> MLKRKQSSRVEAQPVTDFGPDESLSDNADILWINKPWVHSLLRICAIISVISVCMNTPMTFEHYPPLQYVTFTLDTLLMFLYTAEMIAKMHIRGIVKGDSSYVKDRWCVFDGFMVFCLWVSLVLQVFEIADIVDQMSPWGMLRIPRPLIMIRAFRIYFRFELPRTRITNILKRSGEQIWSVSIFLLFFLLLYGILGVQMFGTFTYHCVVNDTKPGNVTWNSLAIPDTHCSPELEEGYQCPPGFKCMDLEDLGLSRQELGYSGFNEIGTSIFTVYEASSQEGWVFLMYRAIDSFPRWRSYFYFITLIFFLAWLVKNVFIAVIIETFAEIRVQFQQMWGTRSSTTSTATTQMFHEDAAGGWQLVAVDVNKPQGRAPACLQKMMRSSVFHMFILSMVTVDVIVAASNYYKGENFRRQYDEFYLAEVAFTVLFDLEALLKIWCLGFTGYISSSLHKFELLLVIGTTLHVYPDLYHSQFTYFQVLRVVRLIKISPALEDFVYKIFGPGKKLGSLVVFTASLLIVMSAISLQMFCFVEELDRFTTFPRAFMSMFQILTQEGWVDVMDQTLNAVGHMWAPLVAIYFILYHLFATLILLSLFVAVILDNLELDEDLKKLKQLKQSEANADTKEKLPLRLRIFEKFPNRPQMVKISKLPSDFTVPKIRESFMKQFIDRQQQDTCCLFRILPSTSSSSCDNPKRPTVEDNKYIDQKLRKSVFSIRARNLLEKETAVTKILRACTRQRMLSGSFEGQPAKERSILSVQHHIRQERRSLRHGSNSQRISRGKSLETLTQDHSNTVRYRNAQREDSEIKMIQEKKEQAEMKRKVQEEELRENHPYFDKPLFIVGREHRFRNFCRVVVRARFNASKTDPVTGAVKNTKYHQLYDLLGLVTYLDWVMITVTICSCISMMFESPFRRVMHAPTLQIAEYVFVIFMSIELNLKIMADGLFFTPTAVIRDFGGVMDIFIYLVSLIFLCWMPQNVPAESGAQLLMVLRCLRPLRIFKLVPQMRKVVRELFSGFKEIFLVSILLLTLMLVFASFGVQLFAGKLAKCNDPNIIRREDCNGIFRINVSVSKNLNLKLRPGEKKPGFWVPRVWANPRNFNFDNVGNAMLALFEVLSLKGWVEVRDVIIHRVGPIHGIYIHVFVFLGCMIGLTLFVGVVIANFNENKGTALLTVDQRRWEDLKSRLKIAQPLHLPPRPDNDGFRAKMYDITQHPFFKRTIALLVLAQSVLLSVKWDVEDPVTVPLATMSVVFTFIFVLEVTMKIIAMSPAGFWQSRRNRYDLLVTSLGVVWVVLHFALLNAYTYMMGACVIVFRFFSICGKHVTLKMLLLTVVVSMYKSFFIIVGMFLLLLCYAFAGVVLFGTVKYGENINRHANFSSAGKAITVLFRIVTGEDWNKIMHDCMVQPPFCTPDEFTYWATDCGNYAGALMYFCSFYVIIAYIMLNLLVAIIVENFSLFYSTEEDQLLSYNDLRHFQIIWNMVDDKREGVIPTFRVKFLLRLLRGRLEVDLDKDKLLFKHMCYEMERLHNGGDVTFHDVLSMLSYRSVDIRKSLQLEELLAREQLEYTIEEEVAKQTIRMWLKKCLKRIRAKQQQSCSIIHSLRESQQQELSRFLNPPSIETTQPSEDTNANSQDHNTQPESSSQQQLLSPTLSDRGGSRQDAADTGKPQRKIGQWRLPSAPKPISHSVSSVNLRFGGRTTMKSVVCKMNPMPDTASCGSEVKKWWTRQLTVESDESGDDLLDI;> MTRGAWMCRQYDDGLKIWLAAPRENEKPFIDSERAQKWRLSLASLLFFTVLLSDHLWFCAEAKLTRTRDKEHHQQQQQQQQQQQQQQQQQQQQQQRQQQRQRQQQRQRQQEPSWPALLASMGESSPAAQAHRLLSASSSPTLPPSPGGGGGSKGNRGKNNRSRALFLGNSAKPVWRLETCYPQGASSGQCFTVESADAVCARNWSRGAAAGEEQSSRGSRPTPLWNLSDFYLSFCNSYTLWELFSGLSSPSTLNCSLDVVLTEGGEMTTCRQCIEAYQDYDHHAQEKYEEFESVLHKYLQSDEYSVKSCPEDCKIVYKAWLCSQYFEVTQFNCRKTIPCKQYCLEVQTRCPFILPDNDEVIYGGLSSFICTGLYETFLTNDEPECCDIRSEEQTAPRPKGTVDRRDSCPRTSLTVSSATRLCPGRLKLCVLVLILLHTVLTASAAQNSTGLGLGGLPTLEDNSTRED

NALCN channel is a voltage-modulated sodium-selective ion channel. It mediates sodium leak currents that are essential for setting the membrane excitability. Sequence analysis shows NALCN protein shares a similar domain arrangement to the pore subunit of eukaryotic voltage-gated sodium channels NaV or calcium channels CaV. In addition to the NALCN subunit, FAM155, UNC79, and UNC80 subunits are indispensable for the function of NALCN channel.

Here, we describe the structure of rat NALCN and mouse FAM155A in detergent to the resolution of 2.7 Å, which provides enhanced details and additional structural insights into the mechanism of this important channel complex. We prepared the NALCN–FAM155A complex in a buffer with sodium chloride and GDN detergent, mimicking the symmetric sodium solution used in electrophysiology recording. The map quality was sufficient for modeling the stable portions of NALCN and FAM155A which encompass 73% of NALCN and 37% of FAM155A. Interestingly, the arrangements of VS are highly asymmetric, with the voltage sensor of domain I (DI-VS) being the most off-axis. On the extracellular side, the CRD of FAM155A protrudes from the top of the complex into the extracellular space while the two predicted transmembrane helices of FAM155A were invisible, probably due to their flexibility. The CRD of FAM155A binds at the top of the NALCN channel. Extracellular loops of domain I, III, and IV (L5I, L5III, L5IV, and L6IV) in NALCN form a platform for FAM155A binding. Unexpectedly, we found the 1387–1390 region of domain IV has two possible alternative conformations, both of which were modeled in the allowed region in the Ramachandran plot validated by Phenix29. Therefore, the arrangement of charged residues at the HFS layer of NALCN selectivity filter (EEK_, − − + 0) is similar to NaV (DEKA, − − + 0) but different from CaV (EEEE, − − − − ), providing a plausible explanation of the sodium selectivity of NALCN. The gate is tightly sealed by several hydrophobic residues on S6 helices, indicating the current structure represents a non-conductive state.The sigma-1 receptor (σ1R) is a non-opioid transmembrane receptor which has been implicated in many diseases, including neurodegenerative disorders and cancer. The sigma-1 receptor (σ1R) is a small, unique integral membrane receptor that is localized primarily in the endoplasmic reticulum (ER). σ1R responds to a structurally diverse array of synthetic ligands such as (+)-pentazocine (agonist) and haloperidol (antagonist). Published structures of human σ1R reveal its homotrimeric organization of a cupin-fold β-barrel body that contains the ligand binding site, a carboxy-terminal V-shaped two-helix bundle, and a single amino-terminal transmembrane helix, while simulation studies have suggested a ligand entry pathway that is generated by conformational rearrangements of the cupin-fold domain. Here, we present multiple crystal structures, including an open-like conformation, of σ1R from Xenopus laevis. Together with functional binding analysis our data suggest that access to the σ1R ligand binding site is likely achieved by protein conformational changes that involve the carboxy-terminal two-helix bundle, rather than structural changes in the cupin-fold domain.

To further validate the structural integrity of the cysteine mutants of xlσ1R, we solved a structure for the xlσ1R-C179/C203 double mutant (xlσ1RC179/C203-S1RA, 3.80 Å) to ensure that the folding of xlσ1R was not disrupted by the cysteine mutation(s). The xlσ1RC179/C203-S1RA structure was solved in the P21 space group, with 24 protomers in each asymmetric unit. The same homotrimeric organization was observed in xlσ1RC179/C203-S1RA, which resembles closely other xlσ1R structures. The α4/α5 region of xlσ1RC179/C203-S1RA appeared also similar to the closed and the open-like conformations. The xlσ1RC179/C203-S1RA crystals were grown in the presence of PRE084, and S1RA was later soaked in after the crystals had formed. Each protomer of the xlσ1RC179/C203-S1RA structure contained one S1RA molecule in the ligand-binding pocket, which adopts a similar pose to the ligand in the xlσ1Rclosed-S1RA structure. As expected, no disulfide bond was formed between Cys179 and Cys203 in this structure, thus allowing S1RA access to and binding in the ligand-binding site. This result indicates that substitution of the residues 179 and 203 with cysteine did not perturb the structural integrity of xlσ1R, and the resulting xlσ1R mutants retained the ligand-binding activity. However, interestingly, in one of the 24 protomers of the xlσ1RC179/C203-S1RA structure, an extra electron density resembling the shape of S1RA was observed near the ligand entrance in addition to the S1RA molecule in the ligand-binding site. The density was readily and best modeled with an S1RA molecule.

>[24x]SVDTMALWLGLRAVLVVAGLAVLLQLIRGWLSSKSYVFNREEIARLAKEHSGLDYEVAFSKIIVELRKKHPGHILQDEDLQWVFVNAGGWMGSMCLLHASLTEYVLLFGTAVDTGGHSGRYWAEISDTILSGTFRQWKEGTTKSEIFYPGDTIVHEVGEATSVQWSSGTWMVEYGRGFIPSTCAFALADTIFSTQDFLTLFYTVKVCSKALLLEASTHLSQLGFF>[4x]MATNEDQKQTESGRHQEVGHKSLLQSDALYQYILETSVFPREHEAMKELREVTAKHPWNIMTTSADEGQFLSMLLKLINAKNTMEIGVYTGYSLLA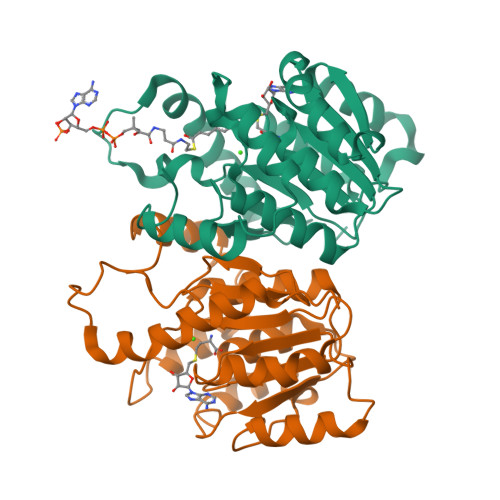TALAIPEDGKILAMDINKENYELGLPVIKKAGVDHKIDFREGPALPVLDEMIKDEKNHGSYDFIFVDADKDNYLNYHKRLIDLVKVGGVIGYDNTLWNGSVVAPPDAPLRKYVRYYRDFVLELNKALAVDPRIEICMLPVGDGITICRRIK(2S)-N,2-dicyclohexyl-2-{5,6-difluoro-2-[6-(1H-pyrazol-1-yl)pyridin-3-yl]-1H-benzimidazol-1-yl}acetamide | C29 H32 F2 N6 O | 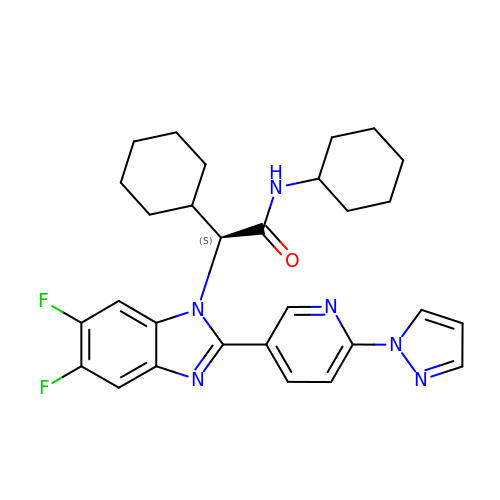BAGJAPIDXZLKQM-MHZLTWQESA-N>MKMLLIHSDYLEFEAKEKTKIAEETENLKGKLDECLACFIAVEREDENNPEGTAIGAVEEIEKVANQLKVNNIVVYPYAHLSSDLSSPETAVKVLKDIESILKERGYNVLRAPFGWYKAFKISCKGHPLSELSRKIVAKEE[6x]

We have been interested in a D-aminoacyl-tRNA deacylase (DTD) fold that is present across the domains of life in two different functional contexts: as an N-terminal editing domain (NTD) of archaeal ThrRS, which specifically removes non-cognate L-serine mischarged on tRNAThr, and as a freestanding ‘chiral proofreading' enzyme, which removes D-amino acids from tRNAs in bacteria and eukaryotes. Both share a striking structural and mechanistic similarity highlighting a common ancestry. Here we show, with the help of structural, biochemical and biophysical studies from three distant organisms, that the substrate specificity in this domain is determined by a differential remodelling of the catalytic centre at the RNA–protein interface rather than just the presence or absence of catalytic water as previously proposed. While demonstrating that the tRNA provides the catalytic group, we show that the side chains within the recognition site are dispensable for the proofreading function, suggesting a primordial mode of protein- or peptide scaffold-based enzymatic activity evolved alongside that of RNA.

To understand this intriguing mechanism of cognate substrate rejection in NTD, we have solved high-resolution crystal structures of ApNTD, as well as NTD from Methanococcus jannaschii (MjNTD) in complex with non-cognate and cognate substrate analogues L-seryl-3′-aminoadenosine (L-Ser3AA) and L-threonyl-3′-aminoadenosine (L-Thr3AA), respectively. In the case of MjNTD, L-Ser3AA and L-Thr3AA complex were crystallized in C2 and P21 space groups with six and four monomers, respectively, in the asymmetric unit corresponding to three and two dimers. However, a clear and complete ligand density was observed in only chain A in the case of MjNTD co-crystals and therefore only this monomer was used for analysis. The possible reason for this could be the remarkably low binding affinity for the ligand in MjNTD, as revealed by binding studies later in this section. L-Ser3AA tightly binds in the active-site pocket in such a way that a conserved hydrogen bond with the main-chain N atom of Lys121 (residue number corresponding to PabNTD) fixes the β-OH group of the substrate in all three NTDs. The carbonyl oxygen of the substrate has a water-mediated interaction with His83 in PabNTD, while the same atom interacts directly with the corresponding His77 in ApNTD and His84 in MjNTD. However, in ApNTD, it has only a water-mediated interaction with the corresponding Glu129, whereas in the case of MjNTD, this group is directly recognized by both Glu135 and His84. Moreover, the catalytic sites in PabNTD and MjNTD accommodate a single water molecule, which is the putative catalytic water Wat1. We also performed biochemical studies with MjNTD against L-Ser-(Ec)tRNAThr and L-(Ec)Thr-tRNAThr to ensure that this enzyme is efficient in non-cognate/cognate discrimination.>TADELVFFVNGKKVVEKNADPETTLLAYLRRKLGLRGTKLGCGEGGCGACTVMLSKYDRLQDKIIHFSANACLAPICTLHHVAVTTVEGIGSTKTRLHPVQERIAKSHGSQCGFCTPGIVMSMYTLLRNQPEPTVEEIEDAFQGNLCRCTGYRPILQGFRTFAK[2x];>[2x]PKQLRFEGERVTWIQASTLKELLDLKAQHPEAKLVVGNTEIGIEMKFKNQLFPMIICPAWIPELNAVEHGPEGISFGAACALSSVEKTLLEAVAKLPTQKTEVFRGVLEQLRWFAGKQVKSVASLGGNIITASPISDLNPVFMASGTKLTIVSRGTRRTVPMDHTFFPSYRKTLLGPEEILLSIEIPYSREDEFFSAFKQASRREDDIAKVTCGMRVLFQPGSMQVKELALCYGGMADRTISALKTTQKQLSKFWNEKLLQDVCAGLAEELSLSPDAPGGMIEFRRTLTLSFFFKFYLTVLKKLG;>DTVGRPLPHLAAAMQASGEAVYCDDIPRYENELFLRLVTSTRAHAKIKSIDVSEAQKVPGFVCFLSADDIPGSNETGLFNDETVFAKDTVTCVGHIIGAVVADTPEHAERAAHVVKVTYEDLPAIITIEDAIKNNSFYGSELKIEKGDLKKGFSEADNVVSGELYIGGQDHFYLETHCTIAIPKGEEGEMELFVSTQNAMKTQSFVAKMLGVPVNRILVRVKRMGGGFGGKETRSTLVSVAVALAAYKTGHPVRCMLDRNEDMLITGGRHPFLARYKVGFMKTGTIVALEVDHYSNAGNSRDLSHSIMERALFHMDNCYKIPNIRGTGRLCKTNLSSNTAFRGFGGPQALFIAENWMSEVAVTCGLPAEEVRWKNMYKEGDLTHFNQRLEGFSVPRCWDECLKSSQYYARKSEVDKFNKENCWKKRGLCIIPTKFGISFTVPFLNQAGALIHVYTDGSVLVSHGGTEMGQGLHTKMVQVASKALKIPISKIYISETSTNTVPNSSPTAASVSTDIYGQAVYEACQTILKRLEPFKKKNPDGSWEDWVMAAYQDRVSLSTTGFYRTPNLGYSFETNSGNA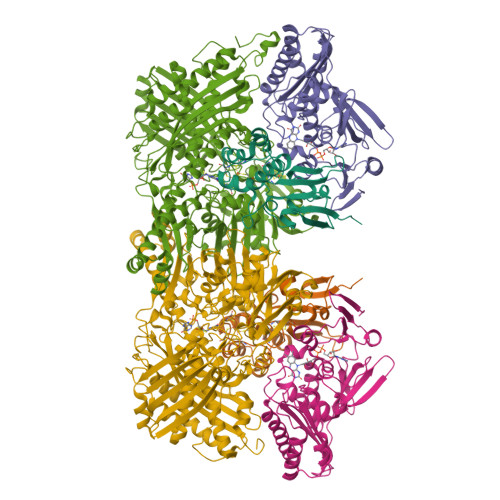FHYFTYGVACSEVEIDCLTGDHKNLRTDIVMDVGSSLNPAIDIGQVEGAFVQGLGLFTLEELHYSPEGSLHTRGPSTYKIPAFGSIPTEFRVSLLRDCPNKKAIYASKAVGEPPLFLGASVFFAIKDAIRAARAQHTNNNTKELFRLDSPATPEKIRNACVDKFTTLCVTGAPGNCK[2x]>STKVVNVAVIGAGVVGSAFLDQLLAMKSTITYNLVLLAEAERSLISKDFSPLNVGSDWKAALAASTTKTLPLDDLIAHLKTSPKPVILVDNTSSAYIAGFYTKFVENGISIATPNKKAFSSDLATWKALFSNKPTNGFVYHEATVGAGLPIISFLREIIQTGDEVEKIEGIFSGTLSYIFNEFSTSQANDVKFSDVVKVAKKLGYTEPDPRDDLNGLDVARKVTIVGRISGVEVESPTSFPVQSLIPKPLESVKSADEFLEKLSDYDKDLTQLKKE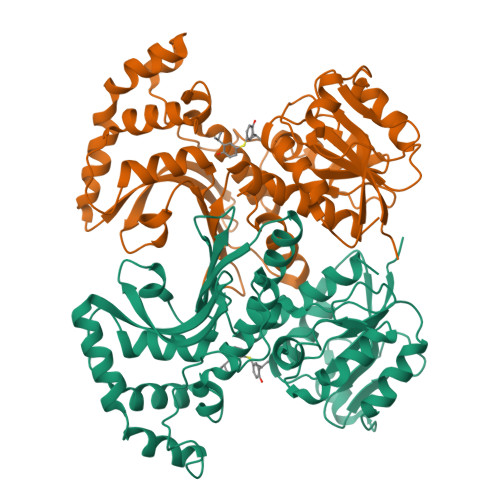AATENKVLRFIGKVDVATKSVSVGIEKYDYSHPFASLKGSDNVISIKTKRYTNPVVIQGAGAGAAVTAAGVLGDVIKIAQRL[2x]> MTRGAWMCRQYDDGLKIWLAAPRENEKPFIDSERAQKWRLSLASLLFFTVLLSDHLWFCAEAKLTRTRDKEHHQQQQQQQQQQQQQQQQQQQQQQRQQQRQRQQQRQRQQEPSWPALLASMGESSPAAQAHRLLSASSSPTLPPSPGGGGGSKGNRGKNNRSRALFLGNSAKPVWRLETCYPQGASSGQCFTVESADAVCARNWSRGAAAGEEQSSRGSRPTPLWNLSDFYLSFCNSYTLWELFSGLSSPSTLNCSLDVVLTEGGEMTTCRQCIEAYQDYDHHAQEKYEEFESVLHKYLQSDEYSVKSCPEDCKIVYKAWLCSQYFEVTQFNCRKTIPCKQYCLEVQTRCPFILPDN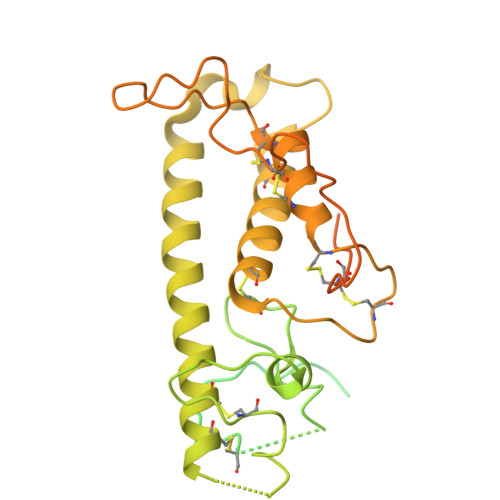DEVIYGGLSSFICTGLYETFLTNDEPECCDIRSEEQTAPRPKGTVDRRDSCPRTSLTVSSATRLCPGRLKLCVLVLILLHTVLTASAAQNSTGLGLGGLPTLEDNSTRED>[2x]MENSSKE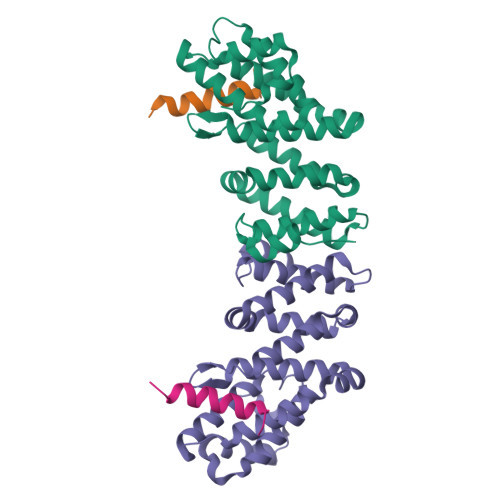DYKIQSFDLETQKLLKTALKDPGSVDLEKVSSVIVDQSLKDQVFSREAGRICYTIVQAEAKQTNGSVFRRNLLNRLQQEFKAREETRKRSTQEWVCLVSFICNIFDYLKVNNMPMVALVHPVYDCLFRLAQSDALKNEEEVDCLVLQLHRIGDQLEKMNVQLMDELFNLLRDGFLLQEDLSSMGRLLLLEILEFRAGGWKLSDTAQKYYYSEVTD;>MATDSWAQAVDEQEAAAESISTLQISEKEEKP[2x]> MSERAPLVIIGTGLAGYNLAREWRKLDGETPLLMITADDGRSYSKPMLSTGFSKNKDADGLAMAEPGAMAEQLNARILTHTR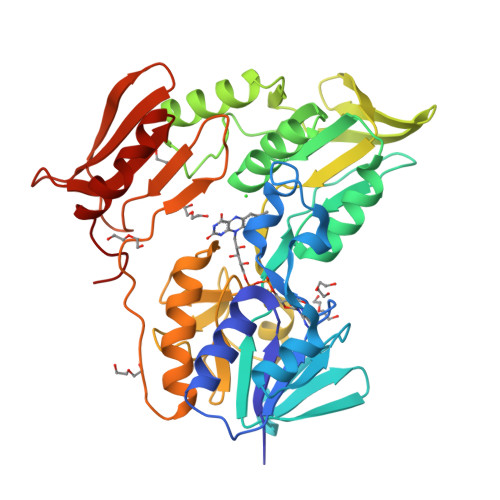VTGIDPGHQRIWIGEEEVRYRDLVLAWGAEPIRVPVEGDAQDALYPINDLEDYARFRQAAAGKRRVLLLGAGLIGCEFANDLSSGGYQLDVVAPCEQVMPGLLHPAAAKAVQAGLEGLGVRFHLGPVLASLKKAGEGLEAHLSDGEVIPCDLVVSAVGLRPRTELAFAAGLAVNRGIVVDRSLRTSHANIYALGDCAEVDGLNLLYVMPLMACARALAQTLAGNPSQVAYGPMPVTVKTPACPLVVSPPPRGMDGQWLVEGSGTDLKVLCRDTAGRVIGYALTGAAVNEKLALNKELPGLMA>[2x]MYLSKVIIARAWSRDLYQLHQGLWHLFPNRPDAARDFLFHVEKRNTPEGCHVLLQSAQMPVSTAVATVIKTKQVEFQLQVGVPLYFRLRANPIKTILDNQKRLDSKGNIKRCRVPLIKEAEQIAWLQRKLGNAARVEDVHPISERPQYFSGDGKSGKIQTVCFEGVLTINDAPALIDLVQQGIGPAKSMGCGLLSLAPL;>MSNFINIHVLISHSPSCLNRDDMNMQKDAIFGGKRRVRISSQSLKRAMRKSGYYAQNIGESSLRTIHLAQLRDVLRQKLGERFDQKIIDKTLALLSGKSVDEAEKISADAVTPWVVGEIAWFCEQVAKAEADNLDDKKLLKVLKEDIAAIRVNLQQGVDIALSGRMATSGMMTELGKVDGAMSIAHAITTHQVDSDIDWFTAVDDLQEQGSAHLGTQEFSSGVFYRYANINLAQLQENLGGASREQALEIATHVVHMLATEVPGAKQRTYAAFNPADMVMVNFSDMPLSMANAFEKAVKAKDGFLQPSIQAFNQYWDRVANGYGLNGAAAQFSLSDVDPITAQVKQMPTLEQLKSWVRNNGEA[12x];>MRSYLILRLAGPMQAWGQPTFEGTRPTGRFPTRSGLLGLLGACLGIQRDDTSSLQALSESVQFAVRCDELILDDRRVSVTGLRDYHTVLGAREDYRGLKSHETIQTWREYLCDASFTVALWLTPHATMVISELEKAVLKPRYTPYLGRRSCPLTHPLFLGTCQASDPQKALLNYEPVGGDIYSEESVTGHHLKFTARDEPMITLPRQFASREWYVIKGGMDVSQ[2x];>[2x]MNLLIDNWIPVRPRNGGKVQIINLQSLYCSRDQWRLSLPRDDMELAALALLVCIGQIIAPAKDDVEFRHRIMNPLTEDEFQQLIAPWIDMFYLNHAEHPFMQTKGVKANDVTPMEKLLAGVSGATNCAFVNQPGQGEALCGGCTAIALFNQANQAPGFGGGFKSGLRGGTPVTTFVRGIDLRSTVLLNVLTLPRLQKQFPNESHTENQP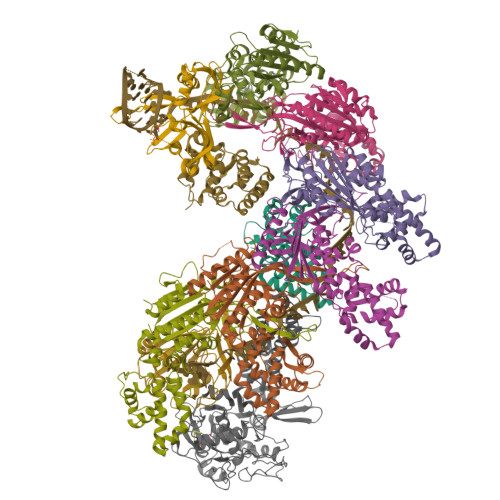TWIKPIKSNESIPASSIGFVRGLFWQPAHIELCDPIGIGKCSCCGQESNLRYTGFLKEKFTFTVNGLWPHPHSPCLVTVKKGEVEEKFLAFTTSAPSWTQISRVVVDKIIQNENGNRVAAVVNQFRNIAPQSPLELIMGGYRNNQASILERRHDVLMFNQGWQQYGNVINEIVTVGLGYKTALRKALYTFAEGFKNKDFKGAGVSVHETAERHFYRQSELLIPDVLANVNFSQADEVIADLRDKLHQLCEMLFNQSVAPYAHHPKLISTLALARATLYKHLRELKPQGGPSNG;>[4x]GPGYQMADEIDAMALYRAWQQLDNGSCAQIRRVSEPDELRDIPAFYRLVQPFGWENPRHQQALLRMVFCLSAGKNVIRHQDKKSEQTTGISLGRALANSGRINERRIFQLIRADRTADMVQLRRLLTHAEPVLDWPLMARMLTWWGKRERQQLLEDFVLTTNKNA>SKPKAVIFDVDGTLAKMNGRGPYDLEKCDTDVINPMVVELSKMYALMGYQIVVVSGRESGTKEDPTKYYRMTRKWVEDIAGVPLVMQCQREQGDTRKDDVVKEEIFWKHIAPHFDVKL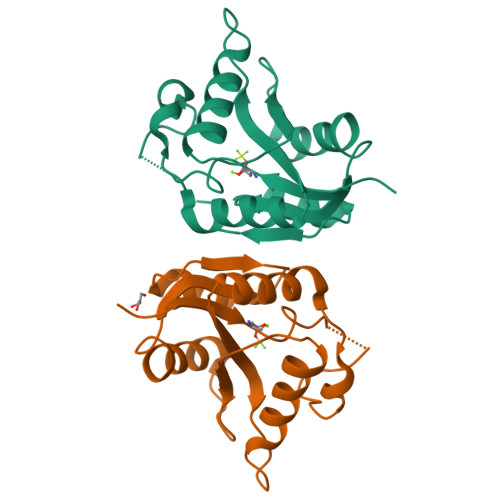AIDDRTQVVEMWRRIGVECWQVASGDF[2x]>MKYILVTGGVISGIGKGIIASSIGTILKSCGLRVTAIKIDPYINIDAGTFSPYEHGEVFVLNDGGEVDLDLGNYERFLDINLYKDNNITTGKIYQHVINKERRGDYLGKTVQVVPHITDAVQEWVMNQAKVPVDGNKEEPQICVIELGGTIGDIEGMPFVEAFRQFQFKAKRENFCNIHVSLVPQLSATGEQKTKPTQNSVRALRGLGLSPDLIVCRSSTPIEMAVKEKISMFCHVNPEQVICIHDVSSTYRVPVLLEEQSIVKYFKERLHLPIGDSASNLLFKWRNMADRYERLQKICSIALVGKYTKLRDCYASVFKALEHSALAINHKLNLMYIDSIDLEKITETEDPVKFHEAWQKLCKADGILVPGGFGIRGTLGKLQ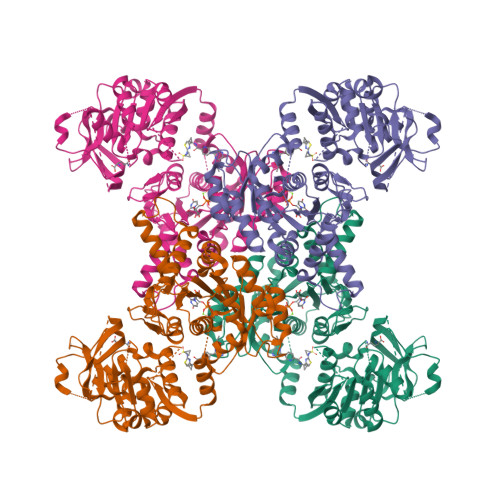AISWARTKKIPFLGVCLGMQLAVIEFARNCLNLKDADSTEFRPNAPVPLVIDMPEHNPGNLGGTMRLGIRRTVFKTENSILRKLYGDVPFIEERHRHRFEVNPNLIKQFEQNDLSFVGQDVDGDRMEIIELANHPYFVGVQFHPEFSSRPMKPSPPYLGLLLAATGNLNAYLQQGCKLSSSDRYSDASDDSFSEPRIAELEIS[4x]> TVTKVSLPEGSFKRVKPQYDEIHIPAPSKPVIDYELKEITSLPDWCQEAFPSSETTSLNPIQSKVFHAAFEGDSNMLICAPTGSGKTNIALLTVLKALSHHYNPKTKKLNLSAFKIVYIAPLKALVQEQVREFQRRLAFLGIKVAELTGDSRLSRKQIDETQVLVSTPEKWDITTRNSNNLAIVELVRLLIIDEIHLLHDDRGPVLESIVARTFWASKYGQEYPRIIGLSATLPNYEDVGRFLRVPKEGLFYFDSSFRPCPLSQQFCGIKERNSLKKLKAMNDACYEKVLESINEGNQIIVFVHSRKETSRTATWLKNKFAEENITHKLTKNDAGSKQILKTEAANVLDPSLRKLIESGIGTHHAGLTRSDRSLSEDLFADGLLQVLVCTATLAWGVNLPAHTVIIKGTDVYSPEKGSWEQLSPQDVLQMLGRAGRPRYDTFGEGIIITDQSNVQYYLSVLNQQLPIESQFVSKLVDNLNAEVVAGNIKCRNDAVNWLAYTYLYVRMLASPMLYKVPDISSDGQLKKFRESLVHSALCILKEQELVLYDAENDVIEATDLGNIASSFYINHASMDVYNRELDEHTTQIDLFRIFSMSEEFKYVSVRYEEKRELKQLLEKAPIPIREDIDDPLAKVNVLLQSYFSQLKFEGFALNSDIVFIHQNAGRLLRAMFEICLKRGWGHPTRMLLNLCKSATTKMWPTNCPLRQFKTCPVEVIKRLEASTVPWGDYLQLETPAEVGRAIRSEKYGKQVYDLLKRFPKMSVTCNAQPITRSVMRFNIEIIADWIWDMNVHGSLEPFLLMLEDTDGDSILYYDVLFITPDIVGHEFTLSFTYELKQHNQNNLPPNFFLTLISENWWHSEFEIPVSFNGFKLPKKFPPPTPLLENISISTSELGNDDFSEVFEFKTFNKIQSQVFESLYNSNDSVFVGSGKGTGKTAMAELALLNHWRQNKGRAVYINPSGEKIDFLLSDWNKRFSHLAGGKIINKLGNDPSLNLKLLAKSHVLLATPVQFELLSRRWRQRKNIQSLELMIYDDAHEISQGVYGAVYETLISRMIFIATQLEKKIRFVCLSNCLANARDFGEWAGMTKSNIYNFSPSERIEPLEINIQSFKDVEHISFNFSMLQMAFEASAAAAGNRNSSSVFLPSRKDCMEVASAFMKFSKAIEWDMLNVEEEQIVPYIEKLTDGHLRAPLKHGVGILYKGMASNDERIVKRLYEYGAVSVLLISKDCSAFACKTDEVIILGTNLYDGAEHKYMPYTINELLEMVGLASGNDSMAGKVLILTSHNMKAYYKKFLIEPLPTESYLQYIIHDTLNNEIANSIIQSKQDCVDWFTYSYFYRRIHVNPSYYGVRDTSPHGISVFLSNLVETCLNDLVESSFIEIDDTEAEVTAEVNGGDDEATEIISTLSNGLIASHYGVSFFTIQSFVSSLSNTSTLKNMLYVLSTAVEFESVPLRKGDRALLVKLSKRLPLRFPEHTSSGSVSFKVFLLLQAYFSRLELPVDFQNDLKDILEKVVPLINVVVDILSANGYLNATTAMDLAQMLIQGVWDVDNPLRQIPHFNNKILEKCKEINVETVYDIMALEDEERDEILTLTDSQLAQVAAFVNNYPNVELTYSLNNSDSLISGVKQKITIQLTRDVEPENLQVTSEKYPFDKLESWWLVLGEVSKKELYAIKKVTLNKETQQYELEFDTPTSGKHNLTIWCVCDSYLDADKELSFEINVK;> SKNEWRKSAIANTLLYLRLKNIYVSADDFVEEQNVYVLPKNLLKKFIEISDVKIQVAAFIYGMSAKDHPKVKEIKTVVLVPQLGHVGSVQISNIPDIGDLPDTEGLELLGWIHTQTEELKFMAASEVATHSKLFADKKRDCIDISIFSTPGSVSLSAYNLTDEGYQWGEENKDIMNVLSEGFEPTFSTHAQLLLSDRITGNFIIPSGNVWNYTFMGTAFNQEGDYNFKYGIPLEFYNEMHRPVHFLQF

The U5 small nuclear ribonucleoprotein particle (snRNP) helicase Brr2 disrupts the U4/U6 small nuclear RNA (snRNA) duplex and allows U6 snRNA to engage in an intricate RNA network at the active center of the spliceosome. The Jab1/MPN domain from the C terminus of Prp8 (Pena et al., 2007; Zhang et al., 2007) forms a complex with Brr2 and strongly stimulates its helicase activity (Maeder et al., 2009; Mozaffari-Jovin et al., 2012). The Brr2 sequence showed an N-terminal region (∼470 amino acids) of unknown function and two consecutive helicase cassettes, each containing a helicase core with two RecA domains followed by a Sec63 unit. Here, we present the structure of yeast Brr2 in complex with the Jab1/MPN domain of Prp8, which stimulates Brr2 activity.

Yeast Brr2 truncated at the N terminus (residues 442–2163) was crystallized together with the Jab1/MPN domain of yeast Prp8 (residues 2147–2413). The structure has been refined at 3.1 Å resolution to Rwork/Rfree of 21.4%/27.0% with excellent stereochemistry. The yeast Brr2 (yBrr2) in the Jab1/MPN domain complex is similar in architecture to the free human Brr2 (hBrr2) with Cα root-mean-square deviation of 2.8 Å for 1,545 aligned residues out of 1,707 residues of yBrr2, both consisting of two structurally similar helicase cassettes forming a compact entity (Santos et al., 2012). Each helicase cassette is composed of six domains: two RecA domains followed by WH, ratchet, helix-loop-helix (HLH), and FN3 domains; the latter three domains are collectively referred to as a Sec63 unit (Pena et al., 2009; Zhang et al., 2009). However, in the C-terminal cassette, there is good density for Mg2+-ADP bound to the Q-loop (residues 1348–1356) and motif I (residues 1372–1377), whereas in the N-terminal cassette, no bound nucleotide was observed. The Jab1/MPN domain (residues 2147–2413) of Prp8 interacts with the ratchet and FN3 domains of the N-terminal Sec63 unit (residues 1011–1309), burying 1,536 Å2 of solvent-accessible surface. The N- and C-terminal helices of the Jab1/MPN domain are gathered to the same side that covers the bottom face of the Sec63 unit. In contrast, in our Brr2-Jab1/MPN complex structure, the C-terminal tail folds into a helical conformation at the interface with the ratchet and HLH domains. Superposition of the Jab1/MPN domain in Brr2-Jab1/MPN and Prp8885–2413-Aar2 complex structures revealed a steric clash between the RNaseH-like domain of Prp8 and Brr2, which accounts for the mutual exclusivity of Aar2 and Brr2 (Galej et al., 2013). The structure accounts for the reduced binding of these pathological mutant Jab1/MPN domains to Brr2 (Maeder et al., 2009), and therefore, it provides detailed insight into the molecular pathology of RP13.>MPFITVGQENSTSIDLYYEDHGTGTPVVLIHGFPLSGHSWERQSAALLDAGYRVITYDRRGFGQSSQPTTGYDYDTFAADLNTVLETLDLQDAVLVGFSMGTGEV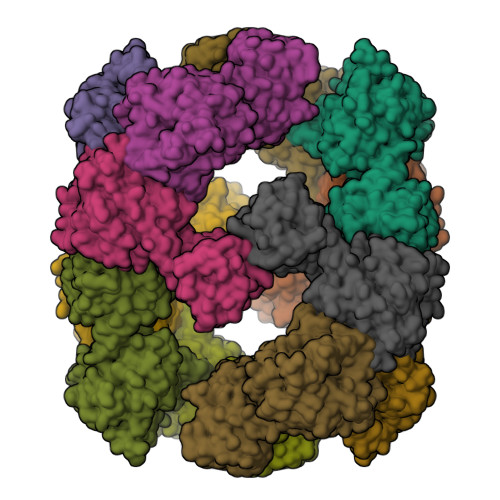ARYVSSYGTARIAAVAFLASLEPFLLKTDDNPDGAAPQEFFDGIVAAVKADRYAFYTGFFNDFYNLDENLGTRISEEAVRNSWNTAASGGFFAAAAAPTTWYTDFRADIPRIDVPALILHGTGDRTLPIENTARVFHKALPSAEYVEVEGAPHGLLWTHAEEVNTALLAFLAKAQEAQKQKLLTEVETYVLSIIPSGPLKAEIAQRLEDVFAGKNTDLEVLMEWLKTRPILSPLTKGILGFVFTLTVPSERGLQRRRFVQNALNGNGDPNNMDKAVKLYRKLKREITFHGAKEISLSYSAGALASCMGLIYNRMGAVTTEVAFGLVCATCEQIADSQHRSHRQLEHHHHHH[3x]Here we report on the discovery of a novel member of this family, pyocin L1 from P. aeruginosa, and show that it utilises lipopolysaccharide (LPS) as a surface receptor, specifically targeting the common polysaccharide antigen (CPA) that is a conserved homopolymer of d-rhamnose. Alignment of the pyocin L1 protein sequence with other lectin-like bacteriocins, LlpA1Pf-5, LlpAPss642, putidacin L1 (LlpABW), LlpAAu1504 from Burkholderia cenocepacia and LlpAXcm761 from Xanthomonas citri pv. malvacearum shows that pyocin L1 contains tandem MMBL domains with three conserved QxDxNxVxY MMBL sugar-binding motifs. Pyocin L1, as predicted by sequence homology to MMBL proteins, consists of two tandem β-prism domains characteristic of MMBLs, connected by antiparallel strands propagating from the end of each MMBL domain and lending a strand to the reciprocal β-prism. In this work we have shown that pyocin L1 targets susceptible cells through binding to the CPA component of LPS and that primary recognition of CPA occurs through binding of d-rhamnose at the conserved QxDxNxVxY sugar binding motifs of the C-terminal lectin domain.

Titration of pyocin L1 into d-rhamnose gave rise to weakly saturable heats of binding that are significantly larger than the heats observed on titration of pyocin L1 into an identical concentration of d-mannose. From this experiment an apparent Kd of 5–10 mM was estimated for the interaction of pyocin L1 with d-rhamnose with apparently weaker binding for d-mannose, Kd>50 mM. In an attempt to determine the location of the pyocin L1 d-rhamnose binding site(s) and the structural basis of the d-rhamnose specificity of pyocin L1 we determined the X-ray structures of pyocin L1 with bound d-mannose, d-rhamnose and in the unbound form. Electron density maps, derived from both d-mannose and d-rhamnose soaked crystals show clear density for sugar moieties in both sites, C1 and C2. The sugars refined well in these densities at full occupancy, giving B-factors comparable to the surrounding protein side chains. The canonical MMBL hydrogen bonds observed for both d-mannose and d-rhamnose were the same: Gln to O3, Asp to O2, Asn to O2 and Tyr to O4. In addition, O6 of d-mannose forms a hydrogen bond with Tyr169 in C1 and His194 in C2. The fact that d-mannose forms an additional hydrogen bond is counter-intuitive given that pyocin L1 has a significantly stronger affinity for d-rhamnose, however Val154, Val163 and Ala166 of C1 and Val184 and Ala191 of C2 form a hydrophobic pocket to accommodate the C6-methyl group of d-rhamnose. Weak density was observed for both sugars at site N1, however given the high concentrations used in the soak and the overall low binding affinity of pyocin L1 for monomeric sugars, it is unlikely that N1 represents a primary binding site for d-rhamnose.

>[2x]MASSLAPRQVIRDGQFITSPNGKYKLVMQADGNLVLYEDGTKPIWNTTPVGPGAKAVMEFNLNLYNKAGQVAWSSNVYTAYLFEEFKDEAYLNLQDDGDFGIFSDEAKWGSIVLSRPEVGVKNKIIPTGTVMVPGTEYINGNYRLAFQGDGNLVIYQINPQVVIWATYTMGADRAVVQEDGNFVIYKGTTALWHTHTATGMPAYLKFTNTGKLFLSQPTLLWTLKRGSLSKPPKVIPGQHGPLDTTPIWSWPHDYPRRRAVVHHHHHH>[2x]MPFTIDTARSIFPETLAADVVPATIARFKQLSAEDQLALIWFAYLEMGKTITIAAPGAANMQFAENTLQEIRQMTPLQQTQAMCDLANRTDTPICRTYASWSPNIKLGFWYELGRFMDQGLVAPIPEGYKLSANANAILVTIQGIDPGQQITVL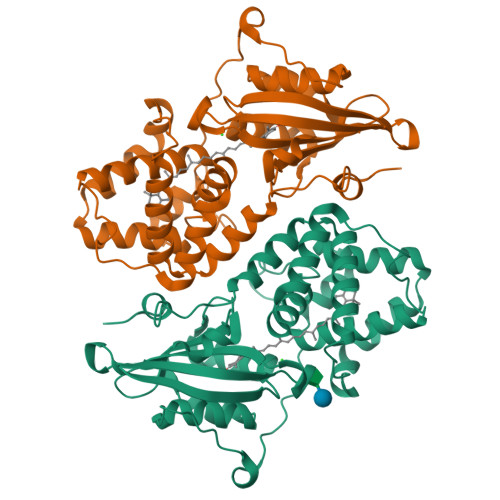RNCVVDMGFDTSKLGSYQRVAEPVVPPQEMSQRTKVQIEGVTNSTVLQYMDNLNANDFDNLISLFAEDGALQPPFQKPIVGKENTLRFFREECQNLKLIPERGVSEPTEDGYTQIKVTGKVQTPWFGGNVGMNIAWRFLLNPENKVFFVAIDLLASPKELLNL>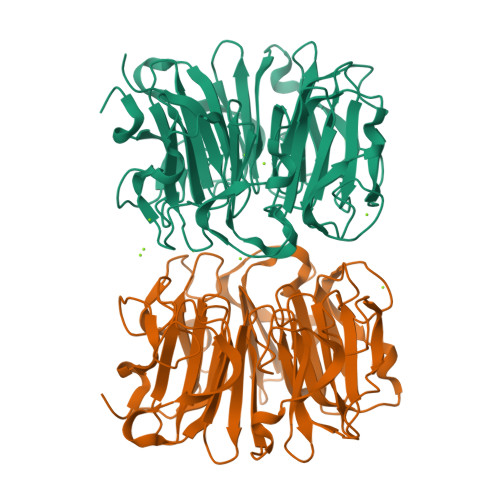[4x]PPRKVLIISAGASHSVALLSGDIVCSWGRGEDGQLGHGDAEDRPSPTQLSALDGHQIVSVTCGADHTVAYSQSGMEVYSWGWGDFGRLGHGNSSDLFTPLPIKALHGIRIKQIACGDSHCLAVTMEGEVQSWGRNQNGQLGLGDTEDSLVPQKIQAFEGIRIKMVAAGAEHTAAVTEDGDLYGWGWGRYGNLGLGDRTDRLVPERVTSTGGEKMSMVACGWRHTISVSYSGALYTYGWSKYGQLGHGDLEDHLIPHKLEALSNSFISQISGGFRHTMALTSDGKLYGWGWNKFGQVGVGNNLDQCSPVQVRFPDDQKVVQVSCGWRHTLAVTERNNVFAWGRGTNGQLGIGESVDRNFPKIIEALSVDGLEHHHHHH>[28x]MMDTQRPLDALGKSINTNVTVYLKDGKLVKGRLKAYDLHMN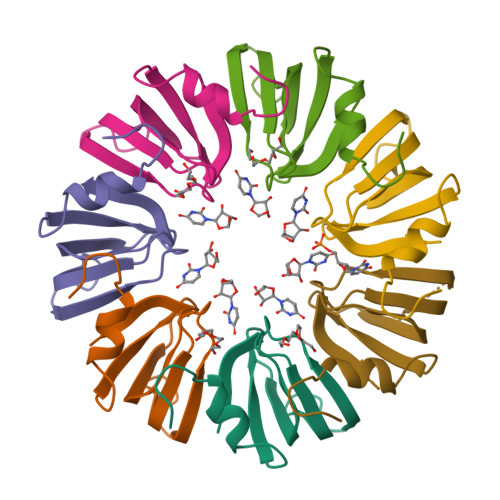VALENAKIESDEEKEFPMLVVRGDNVLYVSL>MISDAMRLIQVALQRYILEFEPELGLSQVVIIENIAMAEELGGQNNQINGHVVMSLVNLQEETTLKNSPHYRLDNGRTIYQNPPVNLNLFILFSALHNQYETSLRLLSRVVEFFQWQKELSFTTTPGIGGISRDLRILPDLYSLTFEQLNHLWGALGGKQVPFVLYRARILSLEAPKRQAEGSTITEIYINE[6x];>MKILYKKILNLELWHDFYLGQPNTPGSLPNNYDISRTLALVPTQECLRVLANLRWVFRPQLYGASLFANVNAAPSGQFPTIFPIDRVYRLTFWLVVSDRYFANFTNLSLINSRNQIYYFSNLSGNEGHALFLTQPLSAYTTNNEYQLGQLVTHADKTLESLTYQGNATNIPNPSDWDSLPASQYVSELDHLPRQGTYRTQVITNANPDNTYNFTLVNTNEQESWAIDVIVPDTHKSGEPFSTSLNFVGQTPGHYRLLENDTQVAEFVLVDNSLPEAFALVEVILNPELVPSAFSLLQASAGQTFIQPKTYVIRFKNRATRWRYRYEQPHGCSAANLPSYFNLIDTHTYATARPIGLRQRPDSLLNDCQDRPLPAPSITLIQPETDGSQRIARIFSDIYL[6x];>MPSTYKTPGVYIEEISKFPPSIAQVETAIPAFIGYTQIAKVGVENFHTDADNLILRPVRITSLLEYEQFFGKAINETTIQVVIQDTTDSRGNLTERKASARITSPSPHNLYYSMQAYFANGGGPCYIVSVGPMSNTGTIQLEALQNGLAEVAKEDEVTLLVFPESQSLSDENYAALMSAALEQCANLQDRFTVMDLKLPATRPIPANAIVGASNAFRDLSLPQDNLKYGACYAPDIETIFNYFYQEDAVTIFRSVNGGAEEQDTLTMAGYNPANGGDGIQYALIESAIDQLPLILPPSPLVVGQYARTDNTRGVWKAPANVALSSVIKPVLKITNEQQNNLNVHPTGKSINAIRAFTGKGTLIWGARTLAGNDNEWRYVSVRRFFNMAEESIKKGSEPFVFEPNDANTWTKVKAMIENFLTLQWRAGALAGAKPEQAFYVKIGLNETMTALDILEGRMIVEIGMAVVRPAEFIILKFSHKMQES[6x];>MAEYPLPKFHFQVDWGGSRLGFTEVSGLDVETEVIEYREGNLPQYHKLKMPGMQKFSNITMKRGTFQGDNDFYKWWNTVALNTIERRDLTISLLNEKHEPVVVWKVNRAWPTKVQSTDLKGDGNEVAIESIEVAHEGLTIQNG[12x]

Contractile injection systems (CISs) are a diverse, yet evolutionarily related, group of assemblies that mediate bacterial cell–cell interactions. Their contractile apparatus is homologous to contractile phage tails, using a contractile outer sheath to propel an effector-loaded tube into target cells. Here, we characterized a CIS in the multicellular cyanobacterium Anabaena, with features distinct from extracellular CISs and T6SSs. In contrast to cytoplasmic free-floating eCISs and cytoplasmic membrane-anchored T6SSs, Anabaena CISs are anchored to the TM, which is mediated by modified tail fibres and a baseplate component.

The resulting maps of the baseplate and of the distal end cap reached resolutions of ~2.9 and ~2.8 Å, respectively. The distal end of the CIS was capped by a tail terminator complex. In contrast to previously studied CISs, the cap of the Anabaena CIS was composed of two proteins, Cis16A and Cis16B, forming a C6-symmetrical complex that terminated the inner tube and sheath, respectively. The structure of the sheath–tube was highly conserved to related CISs and was composed of 23 hexameric layers of the sheath protein Cis2 and 22 hexameric rings of the inner tube protein Cis1. Further details regarding this spike plug and the bipartite cap in a related system are discussed in an accompanying study.To simulate GI bleeding, we utilized an injection-based microfluidics device and found that femtoliter volumes of human serum are sufficient to induce bacterial attraction to the serum source. This response is orchestrated through chemotaxis and the chemoattractant L-serine, an amino acid abundant in serum that is recognized through direct binding by the chemoreceptor Tsr. The full-length Tsr protein includes a periplasmic ligand-binding domain (LBD), a transmembrane HAMP domain, and a cytosolic coiled-coil region, which oligomerizes to form trimers-of-dimers, and complexes with the downstream chemotaxis signaling components, CheA and CheW (Cassidy et al., 2020). We report the first crystal structures of Salmonella Typhimurium Tsr in complex with L-serine and identify a conserved amino acid recognition motif for L-serine shared among Tsr orthologues. The biological distribution of Tsr reveals the chemoreceptor to be widely conserved among Gammaproteobacteria, particularly within the families Enterobacteriaceae, Morganelliaceae, and Yersiniaceae.

To capture a complex with a fully bound ligand site, we grew crystals of the soluble periplasmic portion of the SeTsr LBD with L-serine, at a high salt concentration that would serve as a cryoprotectant without further manipulation, and harvested crystals directly from drops to prevent leaching of the ligand from the binding site. The crystal structure of SeTsr LBD contains five monomers in the asymmetric unit, providing five independent views of the L-serine binding site, with homodimers formed between chains A and B, C and D, and E and its crystal symmetry mate, E′. Lower B-factors in the SeTsr ligand binding region are indicative of greater order, reflecting that our structure is fully serine-bound. SeTsr and EcTsr possess high-sequence similarity in the LBD region—100% identity of the ligand-binding residues and 82.1% identity over the entire periplasmic domain—and as expected, retain a similar global structure with all chains of serine-bound SeTsr, serine-bound EcTsr, and apo EcTsr overlaying within 0.24 Ǻ rmsd over 139 Cα. The higher resolution (+0.3 Ǻ) of the SeTsr structure, and full occupancy of the ligand, provides a much-improved view of the interactions that facilitate specific recognition of L-serine. All five chains of the SeTsr structure are consistent in the positions of the ligand and surrounding residues. Consequently, we can conclude that the correct serine pose and ligand-binding site positions for both models are those we determined using the higher resolution SeTsr structure, in which the L-serine side chain hydroxyl faces outward from the pocket, toward the solvent, and every hydrogen bonding group of the ligand is satisfied by the residues of the binding site.

>[5x]SLKNDKENFTVLQTIRQQQSALNATWVELLQTRNTLNRAGIRWMMDQSNIGSGATVAELMQGATNTLKLTEKNWEQYEALPRDPRQSEAAFLEIKRTYDIYHGALAELIQLLGAGKINEFFDQPTQSYQDAFEKQYMAYMQQNDRLYDIAVEDNNS>MAYRIVSETGDKITVELTLANKNTHYVWNGWCFDIKNITFETTGKVLSIKYADGGEPVYNVNGNLVTIDLTWRGIFHLNTTVKIIIEIQKSGDNPYPHNFKIHYLRGESIIYPTIGELPASWKPGNFTLSDLIADPKSYYDPHVKPHQNGFIMYNPPHPTQIIIGLADIDYPLNLASSARMWVPNKYFAMGLALAYEWFKVNPNFLMALAAKENWGTAVTKDPAFKGYKVIIDEEEYYWPVQIDHPDGIFQVESGNFNQIKAYYPDIFPDTADHDDYMKVS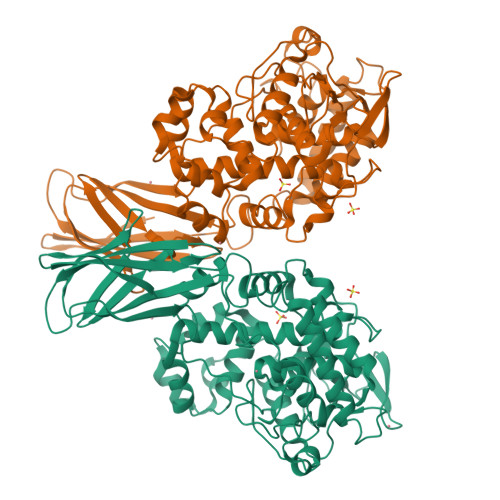LDPNDTAWITSPIVAAVSLTMERELLYAAVGDKYNEFLRLAKDPWAETEIIDFGYNRGVGAIEALKIFSDNWEKAINAEVLWKEFNMEGFGGHVPTVINITATMDMETERIYDANLTWDDIEYFFTVVRQKFFRPGAISDEEWNAMMRDVKRAYDLLSQHWGGDHISYRYDFLTILRVAMKHWPEPHIPRPTGDDWYYHARNYNP[4x]> GSAVSSYRVAEDAREVYDENGNIINLTSKEFDL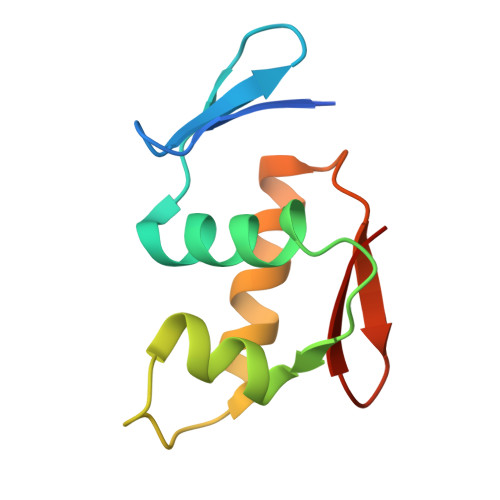LLLFIHHKGHPYSREDILLKVWGHDYFGTDRVVDDLVRRLRRKMPELKVETIYGFGYRMMSS> PDVVLVNGGEPPNPLIPTGTNDSNGGRIIDRLFAGLMSYDAVGKPSLEVAQSIESADNVNYRITVKPGWKFTDGSPVTAHSFVDAWNYGALSTNAQLQQHFFSPIEGFDDVAGAPGDKSRTTMSGLRVVNDLEFTVRLKAPTIDFTLALGHSSFYPLPDSAFRDMAAFGRNPIGNGPYKLADGPAGPAWEHNVRIDLVPNPDYHGNRKPRNKGLRFEFYANLDTAYADLLSGNLDVLDTIPPSALTVYQRDLGDHATSGPAAINQTLDTPLRLPHFGGEEGRLRRLALSAAINRPQICQQIFAGTRSPARDFTARSLPGFDPNLPGNEVLDYDPQRARRLWAQADAISPWSGRYAIAYNADAGHRDWVDAVANSIKNVLGIDAVAAPQPTFAGFRTQITNRAIDSAFRAGWRGDYPSMIEFLAPLFTAGAGSNDVGYINPEFDAALAAAEAAPTLTESHELVNDAQRILFHDMPVVPLWDYISVVGWSSQVSNVTVTWNGLPDYENIVKA;> VVVA

Herein, we show that heme and hemoglobin utilization converge at the cell surface of Mtb after heme is released from hemoglobin and demonstrate that the substrate-binding protein DppA is required for heme uptake across the inner membrane of Mtb. The components of the Mtb Dpp transporter include DppA (R3666c; substrate-binding protein), DppB/C (R3665c/Rv3664c, integral membrane permease proteins), and DppD (Rv3663c, ATPase). The substrate-binding protein DppA associated with the Dpp transporter binds heme with high affinity.

By contrast, the DppAR179A protein was produced in E. coli in similar quantities as wt DppA and was purified to apparent homogeneity with a yield of ~2 mg/l. Surface plasmon resonance experiments and difference absorption spectroscopy showed that heme-binding by DppAR179A was almost completely abolished. The DppAR179A protein yielded crystals of excellent quality that were used to determine the 3D-structure to 1.25 Å resolution. The atomic structure of DppAR179A is identical to wt DppA with an RMSD ~0.11 Å. The observation that mutation of a single amino acid strongly reduced heme binding by DppA without affecting the protein structure demonstrated the specificity of the interaction. Collectively, these experiments showed that arginine 179 is essential for heme binding and identified the heme binding pocket of DppAMtb. To examine the role of heme binding of DppA, we expressed the dpp operon containing wt dppA and dppAR179A in the Mtb Δdpp mutant. While the dpp operon fully restored growth, the dppAR179A gene did not restore growth of the Δdpp mutant with hemin and human hemoglobin as the sole iron sources in HdB minimal medium. We further showed that arginine 179 is essential for heme-binding by DppA in vitro and for Dpp-dependent heme utilization by Mtb.> GIDPFTAKRTHRVINHPYYFPFNGRQAEDYLRSKERGEFVIRQSSRGDDHLVITWKLDKDLFQHIDIQELEKENPLALGKVLIVDNQKYNDLDQIIVEYLQNKVRLLNEMTSSEKFKSGTKKDVVKFIEDYSRVNPNKSVYYFSLNHDNPGWFYLMFKINANSKLYTWNVKLTNTGYFLVNYNYPSVIQLCNGFKTLLKSNSSKNRMNNYR;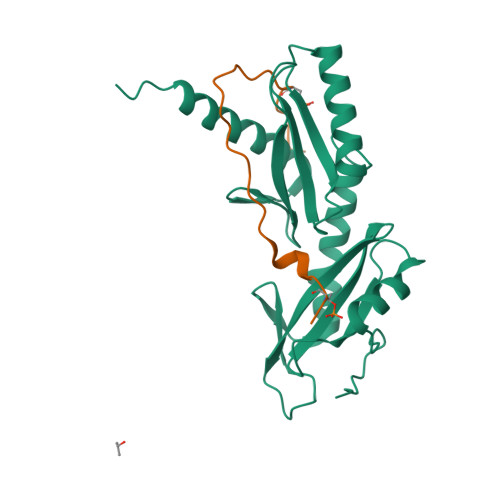> CGGVTPYSNESGLVNADLDVKDELMFSPLVDSGS> MEYKSSPKRPYLLRAYYDWLVDNSFTPYLVVDATYLGVNVPVEYVKDGQIVLNLSASATGNLQLTNDFIQFNARFKGVSRELYIPMGAALAIYARENGDGVMFEPEEIYD;> MEYKSSPKRPYLLRSLYDWLVDNSFTPYLVVDATYLGVNV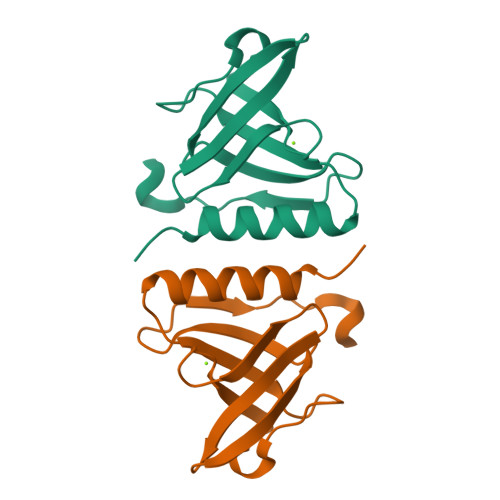PVEYVKDGQIVLNLSASATGNLQLTNDFIQFNARFKGVSRELYIPMGAALAIYARENGDGAMFEPEEIYDE;> MEYKSSPKRPYYLRGFYDWLVDNSFTPYLVVDATYLGVNVPVEYVKDGQIVLNLSASATGNLQLTNDFIQFNQRFKGVSRELYIPMGAALAIYARENGDGMMFEPEEIYDELNIEPDTEQPTGFYEAVD>DVVPHHKLTVNNTKAMKHALERVQLPWKKHSFQEHQSVTSETNTDEHIKDIYDDTERELAFYKQSLDAVLVARDELKRLKVPFKRPLDYFAEMVKSDEHMDKIKGKLIEE[2x];>QFMNKQRTLLISSRGVNYRHRHLIQDLSGLLPHSRKEPKLDTKKDLQQLNEIAELYNCNNVLFFEARKHQDLYLWLSKPPNGPTIKFYIQNLHTMDELNFTGNCLKGSRPVLSFDQRFESSPHYQLIKELLVHNFGVPPNARKSKPFIDHVMSFSIVDDKIWVRTYEISHSTKNKEEYEDGEEDISLVEIGPRFVMTVILILEGSFGGPKIYENKQYVSPNVVRAQIKQQAAEE[2x]

Ribosome assembly is a highly complicated process that engages more than 200 protein assembly factors (AFs) and many snoRNAs. The earliest pre-60S ribosome is co-transcriptionally formed on the 3′ LSU region of pre-rRNA in a stepwise manner. The maturation of pre-60S is coupled to the dynamic association of approximately 90 assembly factors, hierarchical incorporation of RPLs and sequential processing of ITS1 and ITS2. In this study, we determine the cryo-EM structure of pre-60S at an early nucleolar state.

Brx1 is a Brix domain protein that interacts with Ebp2. We determined the crystal structure of Brx1 (residues 26–255) in complex with Ebp2 (residues 195–293) at 2.3 Å resolution with de novo phasing. Brx1 adopts an α/β fold with pseudo 2-fold symmetry, similar to other Brix domain proteins. The structural core of Brx1 is composed of two curved β-sheets that form a half-open β-barrel sandwiching two α-helices (α1 and α3). The surface of the N-terminal sheet holds helix α2, whereas the surface of the C-terminal sheet makes an intermolecular interaction with helix α2′ of Ebp2. In addition, the Ebp2 sequences that flank helix α2′ wrap around the Brx1 structure, forming an extensive interface. In the cryo-EM map, the Brx1-Ebp2 complex perfectly fits into a density bound to domain I. Brx1 interacts with a flat surface formed by H13 and H21. The position of Brx1 would clash with H68 and H88 in domains IV and V in the fully assembled 60S. Thus, the Brx1-Ebp2 complex must be released from the current position for ribosome assembly to proceed.>MTESDVDSGSKKYLSNHKGIFIHVTLEELKRYHQLTPEQKRLIRAIVKTLI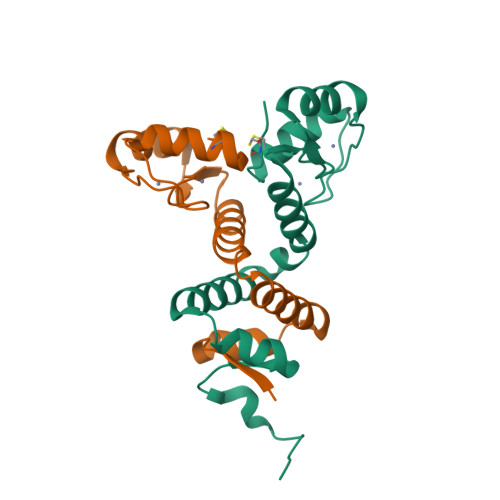HNPQLLDESSYLYRLLASKAISQFVCPLCLMPFSSSVSLKQHIRYTEHTKVCPVCKKEFTSTDSALDHVCKKHNICVS[2x]>MAPSRLCVYCADVCPDRLRCAAWLLATGIFLLLAGCSEAKAPTALERVQKEGVLRVITRNSPATYFQDRNGETGFEYELAKRFAERLGVELKIETADNLDDLYAQLSREGGPALAAAGLTPGREDDASVRYSHTYLDVTPQIIYRNGQQRPTRPEDLVGKRIMVLKGSSHAEQLAELKKQYPELKYEESDAVEVVDLLRMVDVGDIDLTLVDSNELAMNQVYFPNVRVAFDFGEARGLAWALPGGDDDSLMNEVNAFLDQAKKEGLLQRLKDRYYGHVDVLGYVGAYTFTQHLQQRLPRYESHFKQSGKQKDTDWRLLAAIGYQESLWQPGATSKTGVRGLMMLTNRTAQAMGVSNRLDPKQSIQGGSKYFVQIRSELPESIKEPDRSWFALAAYNIGGAHLEDARKMAEKEGLNPNKWLDVKKMLPRLAQKQWYAKTRYGYARGGETVHFV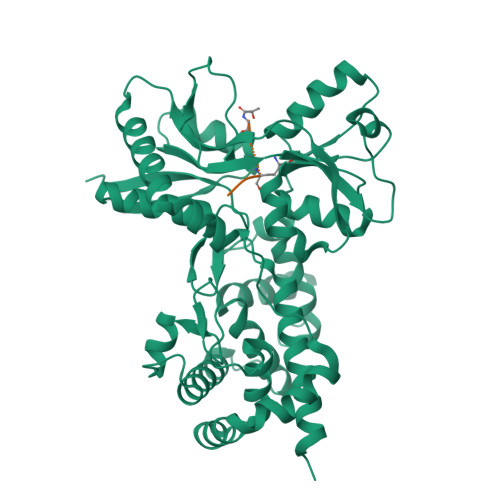QNVRRYYDILTWVTQSQMEGSQIAESGLHLPGVNKTRPEEDSGDEKL[2x];> MAPSRLCVYCADVCPDRLRCAAWLLATGIFLLLAGCSEAKAPTALERVQKEGVLRVITRNSPATYFQDRNGETGFEYELAKRFAERLGVELKIETADNLDDLYAQLSREGGPALAAAGLTPGREDDASVRYSHTYLDVTPQIIYRNGQQRPTRPEDLVGKRIMVLKGSSHAEQLAELKKQYPPLKYEESDAVEVVDLLRMVDVGDIDLTLVDSNELAMNQVYFPNVRVAFDFGEARGLAWALPGGDDDSLMNEVNAFLDQAKKEGLLQRLKDRYYGHVDVLGYVGAYTFTQHLQQRLPRYESHFKQSGKQKDTDWRLLAAIGYQESLWQPGATSKTGVRGLMMLTNRTAQAMGVSNRLDPKQSIQGGSKYFVQIRSELPESIKEPDRSWFALAAYNIGGAHLEDARKMAEKEGLNPNKWLDVKKMLPRLAQKQWYAKTRYGYARGGETVHFVQNVRRYYDILTWVTQPQMEGSQIAESGLHLPGVNKTRPEEDSGDEKL;> MAPSRLCVYCADVCPDRLRCAAWLLATGIFLLLAGCSEAKAPTALERVQKEGVLRVITRNSPATYFQDRNGETGFEYELAKRFAERLGVELKIETADNLDDLYAQLSREGGPALAAAGLTPGRDDDASVRYSHTYLDVTPQIIYRNGQQRPTRPEDLVGKRIMVLKGSSHAEQLAELKKQYPELKYEESDAVEVVDLLRMVDVGDIDLTLVDSNELAMNQVYFPNVRVAFDFGEARGLAWALPGGDDDSLMNEVNAFLDQAKKEGLLQRLKDRYYGHVDVLGYVGAYTFTQHLQQRLPRYESHFKQSGKQKDTDWRLLAAIGYQESLWQPGATSKTGVRGLMMLTNRTAQAMGVSNRLDPKQSIQGGSKYFVQIRSELPESIKEPDRSWFALAAYNIGGAHLEDARKMAEKEGLNPNKWLDVKKMLPRLAQKQWYAKTRYGYARGGETVHFVQNVRRYYDILTWVTQPQMEGSQIAESGLHLPGVNKTRPEEDSGDEKL;> XAEKAA> MSLAEHKGDVMIVDDDAHVRIAVKTILSDAGFHIISADSGGQCIDLLKKGFSGVVLLDIMMPGMDGWDTIRAILDNSLEQGIAIVMLTAKNAPDAKMIGLQEYVVDYITKP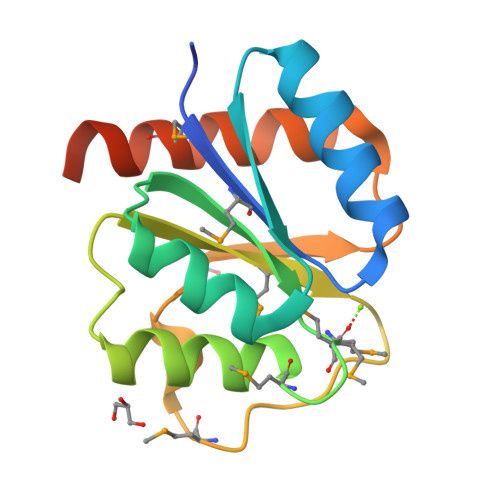FDNEDLIEKTTFFMGFVRNQTGNEGHHHHHH>MMGSDKTVYVVLGGTSGIGAELAKQLESEHTIVHVASRQTGLDISDEKSVYHYFETIGAFDHLIVTAGSYAPAGKVVDVEVTQAKYAFDTKFWGAVLAAKHGARYLKQGGSITLTSGMLSRKVVANTYVKAAINAAIEATTKVLAKELAPIRVNAIS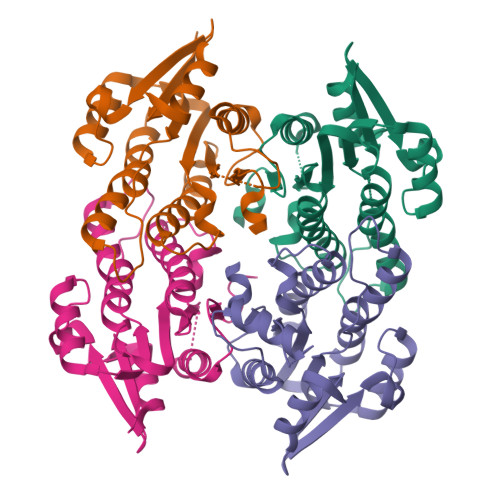PGLTKTEAYKGMNADDRDAMYQRTQSHLPVGKVGEASDIAMAYLFAIQNSYMTGTVIDVDGGALLG[4x]> SMFLPPPECPVFEPSWEEFADPFAFIHKIRPIAEQTGICKVRPPPDWQPPFACDV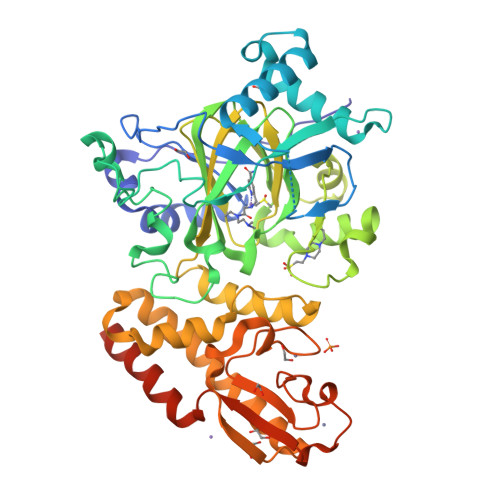DKLHFTPRIQRLNELEAQTRVKLGGGGARDYTLRTFGEMADAFKSDYFNMPVHMVPTELVEKEFWRLVSTIEEDVTVEYGADIASKEFGSGFPVRDGKIKLSPEEEEYLDSGWNLNNMPVMEQSVLAHITADICGMKLPWLYVGMCFSSFCWHIEDHWSYSINYLHWGEPKTWYGVPGYAAEQLENVMKKLAPELFVSQPDLLHQLVTIMNPNTLMTHEVPVYRTNQCAGEFVITFPRAYHSGFNQGFNFAEAVNFCTVDWLPLGRQCVEHYRLLHRYCVFSHDEMICKMASKADVLDVVVASTVQKDMAIMIEDEKALRETVRKLGVIDSERMDFELLPDDERQCVKCKTTCFMSAISCSCKPGLLVCLHHVKELCSCPPYKYKLRYRYTLDDLYPMMNALKLRAESYNEWALNVNEALEAKINK>[6x]MPRGSRSAASRPASRPAAPSAHPPAHPPPSAAAPAPAPSGQPGLMAQMATTAAGVAVGSAVGHVMGSALTGAFSGGSSEPSQPAVQQAPTPAAPQPLQ

Mitochondrial proteins CHCHD10 and CHCHD2 are mutated in rare cases of heritable FTD, ALS and PD and aggregate in tissues affected by these diseases. Here, we demonstrate that the low complexity N-terminal domains of both D10 and D2, as well as the full-length proteins, can form amyloid fibrils in vitro and in vivo. Structures of D10 and D2 fibrils assembled in vitro from the low complexity N-terminal domains of each protein show that their core comprises the most highly conserved region between the two proteins. For D10 and D2, the central conserved VAV motif forms a beta-strand that is associated with the protofilament interface in all the structures we have observed, suggesting that it may be a critical element in fibril formation and may be expected to appear in ex vivo structures as well.

Using cryo-EM, we observed several distinct D10-NT fibril polymorphs (see Methods section on Cryo-EM sample preparation and data collection) and determined three different structures. The first structure we obtained (polymorph-1, 2.31 Å resolution) revealed an ordered core formed by residues P42-G75 and containing two identical protofilaments (PFs) related by pseudo-21 helical screw symmetry. Each PF contains three beta-strands, extending from residues M45 to A53, V55-V57, and V64-A72. Strand-2 forms part of a beta-helix-like turn structure, commonly observed in amyloid fibrils, connecting the first and third strands. The interface between these PFs is formed primarily between the tip of each beta-helix and the N-terminal half of strand 1. Strand-1 adopts a very similar conformation to that observed in the D10-NT PF1 structure, as do the last five residues of strand-3, and the two strands pack together in a nearly identical manner in both structures, with residue F73(D10)/F84(D2) packing against the equivalent Q47(D10)/Q58(D2) residue. Similarly, the location of the equivalent residues in the D10-NT PF1 fold suggests that it could accommodate D2 molecules. In the case of p.G66V, the PF2 or PF3 structures could potentially accommodate the mutation, but it would not be consistent with the PF1 structure and would therefore be expected to eliminate some of the possible WT PF folds.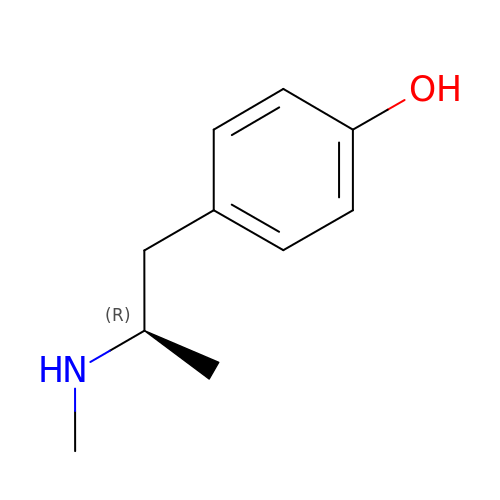4-[(2R)-2-(methylamino)propyl]phenol | C10 H15 N O | SBUQZKJEOOQSBV-MRVPVSSYSA-N> DVSGTVCLSALPPEATDTLNLIASDGPFPYSQDGVVFQNRESVLPTQSYGYYHEYTVITPGARTRGTRRIITGEATQEDYYTGDHYATFSLIDQTC;> KKAVINGEQIRSISDLHQTLKKELALPEYYGENLDALWDCLTGWVEYPLVLEWRQF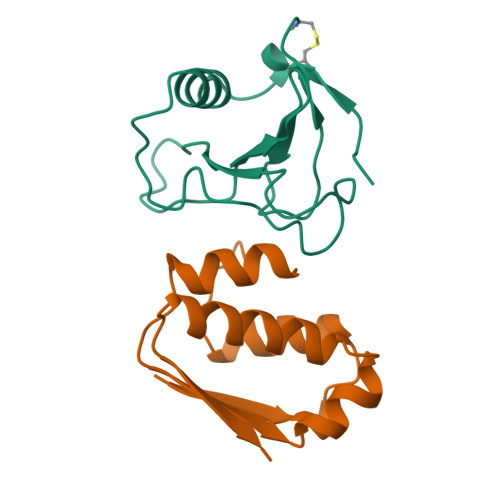EQSKQLTENGAESVLQVFREAKAEGCDITIILS> DSSDEASVSPIADNEREAVTLLLGYLEDKDQLDFYSGGPLKALTTLVYSDNLNLQRSAALAFAEITEKYVRQVSREVLEPILILLQSQDPQIQVAACAALGNLAVNNENKLLIVEMGGLEPLINQMMGDNVEVQCNAVGCITNLATRDDNKHKIATSGALIPLTKLAKSKHIRVQRNATGALLNMTHSEENRKELVNAGAVPVLVSLLSSTDPDVQYYCTTALSNIAVDEANRKKLAQTEPRLVSKLVSLMDSPSSRVKCQATLALRNLASDTSYQLEIVRAGGLPHLVKLIQSDSIPLVLASVACIRNISIHPLNEGLIVDAGFLKPLVRLLDYKDSEEIQCHAVSTLRNLAASSEKNRKEFFESGAVEKCKELALDSPVSVQSEISACFAILALADVSKLDLLEANILDALIPMTFS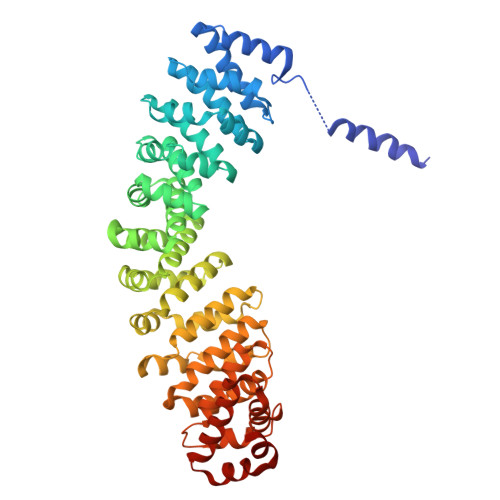QNQEVSGNAAAALANLCSRVNNYTKIIEAWDRPNEGIRGFLIRFLKSDYATFEHIALWTILQLLESHNDKVEDLVKNDDDIINGVRK3-(6-ethoxynaphthalen-2-yl)-1-(propan-2-yl)-1H-pyrazolo[3,4-d]pyrimidin-4-amine | C20 H21 N5 O | 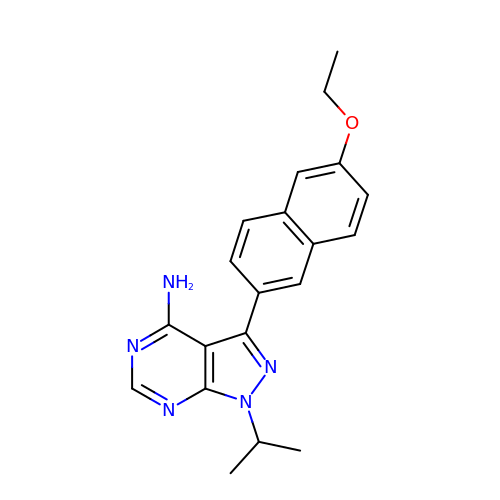MJOCJDMQRCJQJF-UHFFFAOYSA-N>GGGGTGGGA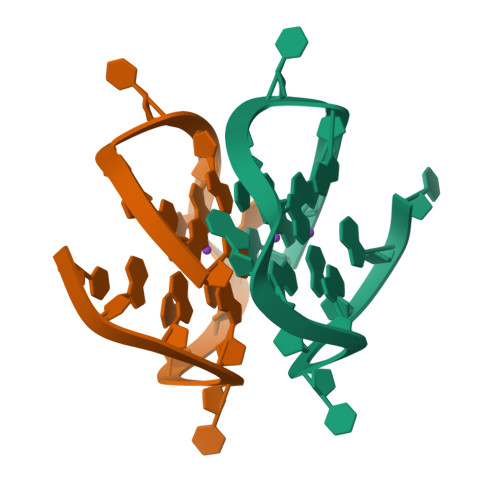GGTGGGT[2x]> DAVGTGISVVGQILGVVGVPFAGALTSFYQSFLNTIWPSDADPWKAFMAQVEVLIDKKIEEYAKSKALAELQGLQNNFEDYVNALNSWKKTPLSLRSKRSQDRIRELFSQAESHFRNSMPSFAVSKFEVLFLPTYAQAANTHLLLLKDAQVFGEEWGYSSEDVAEFYHRQLKLTQQYTDHCVNWYNVGLNGLRGSTYDAWVKFNRFRREMTLTVLDLIVLFPFYDIRLYSKGVKTELTR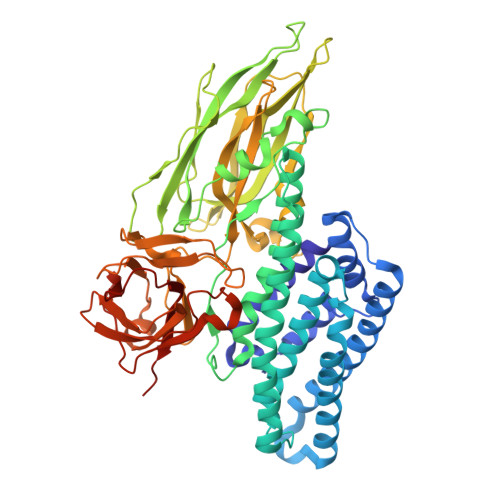DIFTDPIFSLNTLQEYGPTFLSIENSIRKPHLFDYLQGIEFHTRLQPGYFGKDSFNYWSGNYVETRPSIGSSKTITSPFYGDKSTEPVQKLSFDGQKVYRTIANTDVAAWPNGKVYLGVTKVDFSQYDDQKNETSTQTYDSKRNNGHVSAQDSIDQLPPETTDEPLEKAYSHQLNYAECFLMQDRRGTIPFFTWTHRSVDFFNTIDAEKITQLPVVKAYALSSGASIIEGPGFTGGNLLFLKESSNSIAKFKVTLNSAALLQRYRVRIRYASTTNLRLFVQNSNNDFLVIYINKTMNKDDDLTYQTFDLATTNSNMGFSGDKNELIIGAESFVSNEKIYIDKIEFIPVQL>GMQQSEHFSFGEQTEIEDIGGGLKRQMLGFNHELMAVKIWFDKGAEGYVHAHRHSQVSYVVEGEFHVNVDGVIKVLTAGDSFFV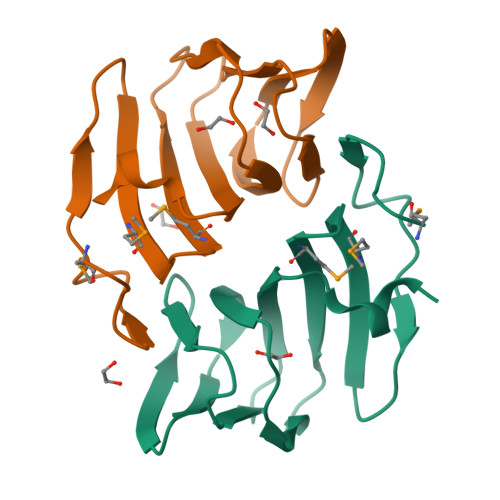PPHVDHGAVCPTGGILIDTFSPAREDFVEGLS[2x]>[4x]NNNGACUU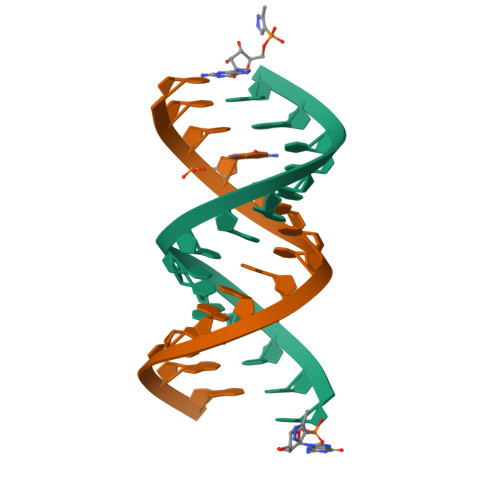AAGUCGG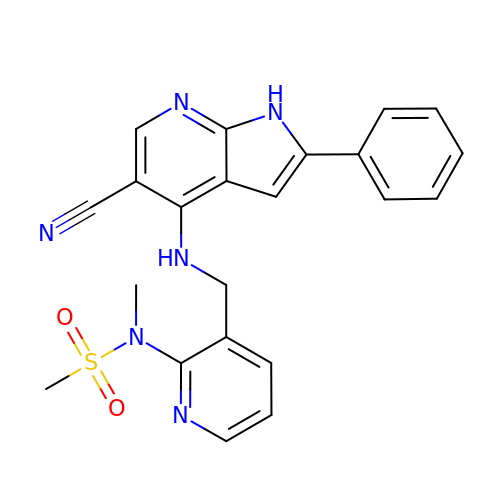N-(3-{[(5-cyano-2-phenyl-1H-pyrrolo[2,3-b]pyridin-4-yl)amino]methyl}pyridin-2-yl)-N-methylmethanesulfonamide | C22 H20 N6 O2 S | IFWXGGDEGREJOB-UHFFFAOYSA-N>PPAIPGIPGIPGT[6x];>[6x]APDGKKGEAGRPG;>[6x]GIPGMPGLPGAPGK

One of the of most well-studied defense collagens is complement component 1q (C1q) found in mammalian serum. A key feature of C1q is its “bouquet” structure, containing six flower-like C-terminal globular domains, an intermediate “branching” collagen-like region, and an N-terminal “stem” where the collagen-like portions bundle together. We have recently recapitulated the unique C1q octadecameric structure in a series of short (∼40 amino acids) synthetic peptides derived from the native sequence of the C1q stem region. Here we use a peptide self-assembly system to design collagenous assemblies based on the C1q collagen-like region.

Then we were able to determine the structure of a small narrow region of the assembly to 3.5 Å resolution from which we were able to build an atomic model. We generated a ∼ 3.5 Å resolution structure of the narrow region of the assembly which resulted in us being able to reliably model the side chains within this region. It should be noted that the molecular weight of the interpretable portion of the narrow region structure was less than 30 kDa. An interesting structural feature we identified in this model is the interweaving of hydroxyproline residues at the interface of peptide B from one PPII trimer and peptide C from another PPII trimer which evokes the “knobs-in-holes” interfaces of α-helical coiled-coils. Such an interaction could not exist in a canonical triple-helical configuration with a right-handed superhelical twist. Further examination of the model revealed that the lumen in the narrow region was dominated by rings of hydrophobic amino acids. Cross sections of the structure revealed that there were three sets of hydrophobic residues, forming rings with identical residues due to the C6 symmetry at isoleucine 7, methionine 10, and leucine 13 of peptide C. The diameter across the cavity formed by the hydrophobic rings was ∼5–6 Å. We are fairly confident in the side chain positioning of Arg16 as that is well-defined in the high-resolution narrow region model.>GQENKKEIINKPLTDSLIVYQTENLIINKLSNHIYEHISFLNTDDFGKVACNGMLVLNENKVVVFDTPTDDKSSLELINFVTNTLKSEIIGLIPTHFHDDCIGGITEFENHNIQTYVSKETIELLKDNGQEFSNPTKDFDNSLTLDIGNKKVYAEYFGEGHTKDNVVGYF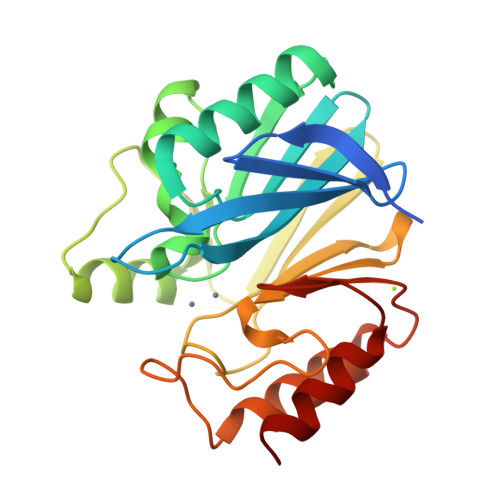PEDNAVFGGCLIKEIDASKGYLGDANIKEWSTTVEKVKLKYPNAKIVIPGHGKWGGIELFDYTIKLFE[2x]>MTSMKKVLTSLAVGIPSPLPPPCKELDESVPHAPKRTPNLSPADRRQAIANALRYFNTADHEVLAEEFSRELDEYGHIYMYRLRPTQYEMRAYPITDYPAKSKYAAAMMMMIMNNLDNRVAMFPHELITYGGNGGVFNNWAQFCLTMKYLCEMTDHQTLALYSGHPLGLFPSHPDAPRAVITNGMMVPNYSTREQYDRLYAMGCTQYGQMTAGSFCYIGPQGIVHGTTITFRNAGRKYLGVEDLAGKVVLTSGLGGMSGAQGKAGVICGAVVVVAEVDPNALYKRKGQGWLMEVETDVEALLRRVRAASAAKEAVSIGFLGNVVTVWERLVKEKDEIVHLGSDQTSCHNPFNGGYYPVQLTFEESKKMMVEDPAMFKELVQESLRRQVAAINEMSARGLRFWDYGNSFLLEASRAGAEVWTPDDTVRSINRFRYPSYVQDIMGDIFALGFGPFRWVCTSCLPEDLELTDRIATETLEKLMKDASTKSQKQISDNLLWIKQAGENKLVVGSQARILYADCEGRQTIAKNFNDAVRDGRLKGPVVLSRDHHDVSGTDSPFRETSDLYDGSSLTADMAVQNVIGDAFRGATWVSLHNGGGTGWGEATNGGFCLVLDGSADAERRA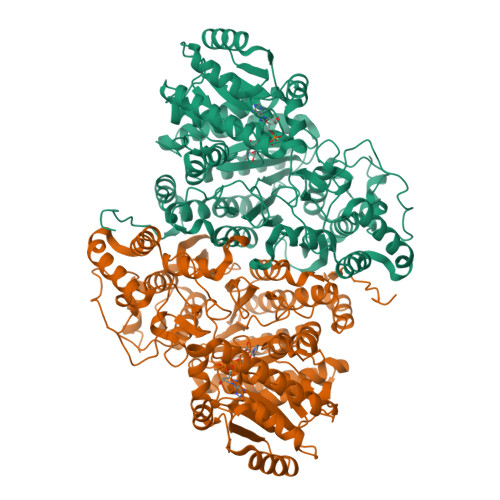KLMLLWDVLNGVTRRAWSGNACGHEAMLRAVSRVEGLHVTVPQHVHPDVLKKYHHHHHH[4x]>[26x]FSGLEAAIVLIAFVVVAAVFSYVMLGAGFFA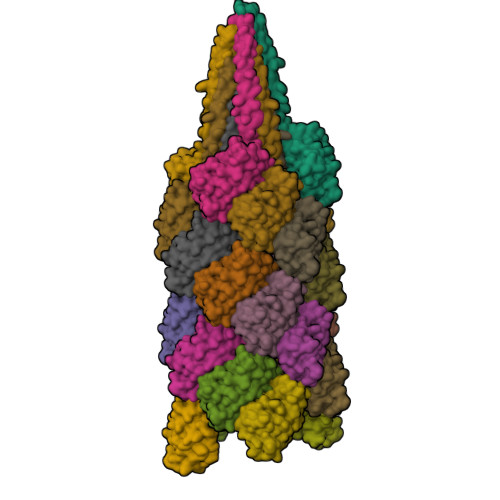TQKSQEVTYSGMKQATSNLILDGMIYGSYSKGGSGLAQLYFYVKVPEGGETQDLKYVTYLWTKENKAVTTLTSITPTNQQLNPGARVKVTITAPTGYKPIAGQKFVLEIKPKTGASTIVTRTLSDGYNGGVII>HHHHHHGSTRTAISRREYDEWLSEAASLARALRYPVTPEMVNDSAGIVFGDDQYEAFAHGLWSREPYEVMVILESLNEPAVDGLPAAGAAHAEYSGLCDKLMIVHPGKFCPPHFHQRKTESYEVVLGEMEVFYAPEPVTVGDDDVLSFSPMPEGSPWPEGVALPAGREDSYAGLTSYVRLRAGDPKFVMHRKHLHAFRCPADSPVPLVVREVSTYSHEPTEHAHDKAAPLPQWRGLHDNTFVAEAANSG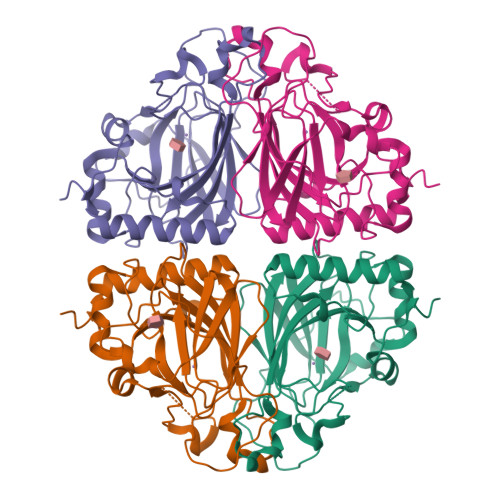RLATAIA[2x]> MQGAEGALTGKQPDGSAEKAVLEQFGFPLTGTEARCYTNHALSYDQAKRVPRWVLEHISKSKIMGDADRKHCKFKPDPNIPPTFSAFNEDYVGSGWSRGHMAPAGNNKFSSKAMAETFYLSNIVPQDFDNNSGYWNRIEMYCRELTERFEDVWVVSGPLTLPQTRGDGKKIVSYQVIGEDNVAVPSHLYKVILARRSSVSTEPLALGAFVVPNEAIGFQPQLTEFQVSLQDLEKLSGLVFFPHLDRTSDIRNICSVDTCKLLDFQEFTLYLSTRKIEGARSVLRLEKIMVNLKNAEIEPDDYFMS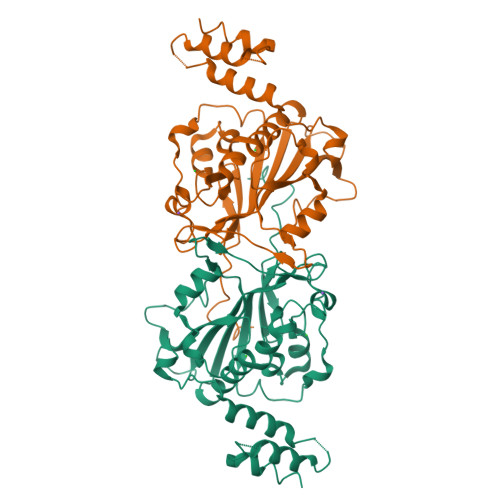RYEKKLEELKAKEQSGTQIRKPSAHHHHHH>GSHMSVPQGAPGDLYVAGCGVWLPPPVTTEQALAAGHCDRRLASSTRMLSVAVADKETPAEMAALAAQTALDRSGVAPAHVDLVLHASLYFQGHHLWAPSSYVQRVAVGNRCPAMEVRQVXNGGMAALELARAYLLAAPDRVAALITTGDRMHPPGFDRWSSDPGTVYADGGTALVLSRQGGFARLRSLVTVSEPVLEGMHRGGHPFGPPSPEEQRAVDLDAHKRAYVAEAGSSFSVARVSAGQEEALTGALEAAGAGLDDISRVVLPHMGWRRLSAAYFNKWHIQPERTTWEFGRRT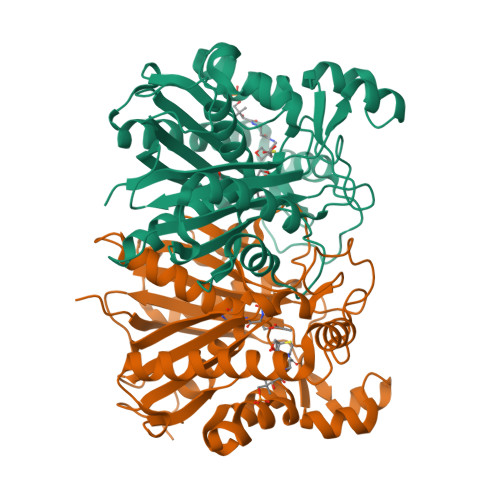GHLGGGDPIAGFDHLVGSGRLAPGELCLLVSVGAGFSWSCAVVELLERPSWAAAPAAR[2x]>GSMSSDAQWLTAEERDQLIPGLKAAGWSELSERDAIYKEFSFKNFNQAFGFMSRVALQAEKMNHHPEWFNVYNKVQITL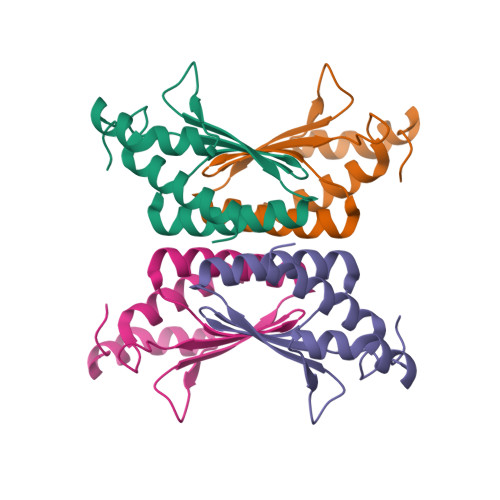TSHDCGGLTKRDVKLAQFIEKAAASL[2x]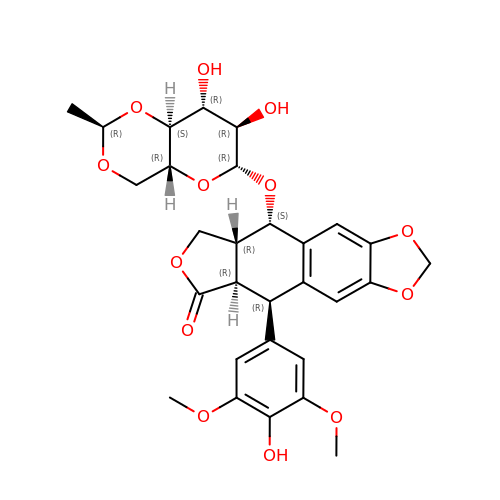(5S,5aR,8aR,9R)-9-(4-hydroxy-3,5-dimethoxyphenyl)-8-oxo-5,5a,6,8,8a,9-hexahydrofuro[3',4':6,7]naphtho[2,3-d][1,3]dioxol-5-yl 4,6-O-[(1R)-ethylidene]-beta-D-glucopyranoside | C29 H32 O13 | VJJPUSNTGOMMGY-MRVIYFEKSA-N>DAGTSNVTVTVSDKDVLLEVQCRWEELLMTRVFDAIKSLHLDVLSVQASAPDGFMGLKIRAQFAGSGAVVPWM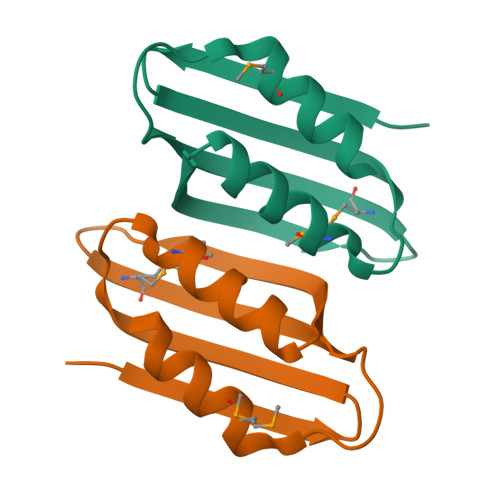ISEALRKAIGKR[2x]> AGHMYNPRCKDLDRDYFPSYHTTRFQDQPEPNLAVLEHFVRVTKQHGRELTEKQGITVDHLRYGEGRQLVDVFYSEKTTNQAPLFVFVHGGYWQEMDMSMSCSIVGPLVRRGYRVAVMDYNLCPQVTLEQLMTQFTHFLNWIFDYTEMTKVSSLTFAGHSAGAHLLAQILMRPNVITAQRSKMVWALIFLCGVYDLRELSNLESVNPKNILGLNERNIESVSPML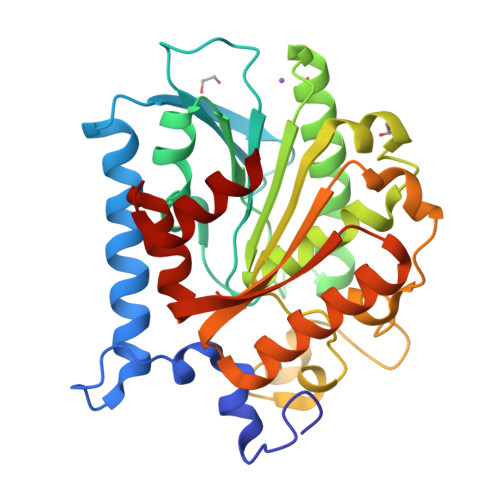WEYTDVTVWNSTKIYVVAAEHDSTTFIEQSRHYADVLRKKGYKASFTLFKGYDHFDIIEETAIDDSDVSRFLRNIEIE> GPLGSEQQPGDRCPRHVARIIAENDPPIRCDLTLQELLSEVQVDFEPSASEVVAMEGLMDEQHFIPHDPHSKKAAVQSLVIAIKTADLLLQMIHENVKRDIRTTCIQMANESYARADIVRDSLIAASQGKYTALGKIVFHSYTNFMPVNANESEKRAWMEMLGECTSHGNKLCEMANAQVEQETRDIINIMFKNIDDVVTQTTRAMRGVFDPPDTVKALSAAAQLIRVWEHDNVINDQSVSTSSVVTAALEANENLAKALRDVSGYAEVQFNRLCLSILTSAKERIDIIYHSARSQHLACNVRMNVAQQNLATFILTNARERPNDAVIRTRRAVANTGILLFTGQHITRDALDKAAESKSVEEIVGMS

To ensure the success of lytic replication, the herpesvirus human cytomegalovirus (HCMV) expresses the immediate-early protein IE1, which acts as an antagonist of antiviral, subnuclear structures termed PML nuclear bodies (PML-NBs). IE1 interacts directly with PML, the key protein of PML-NBs, through its core domain and disrupts the dot-like multiprotein complexes thereby abrogating the antiviral effects. Structural characterization of IE1 has shown that it comprises a folded core domain (IE1CORE), which mediates the interaction with PML and is flanked by a short disordered region at the N-terminus and a longer disordered region at the C-terminus containing a SUMOylation motif and a STAT interaction site. All three IE1CORE proteins display a femur-like structure consisting of α-helices only.

Of the two ratIE1 variants, only the N-terminally truncated variant yielded protein crystals. This variant, covering residues 30 to 392, is from here-on referred to as the ratIE1CORE domain. For crystallization, surface lysine residues of ratIE1 30–392 were chemically methylated. The structure of ratIE1CORE was solved to 3.4 Å resolution with Rwork = 21.5% and Rfree = 24.6%. Initial phases were obtained with the MAD technique since any molecular replacement calculations with the previously determined rhesIE1CORE structure failed. The main chain of ratIE1CORE could be built from residues 33 to 392, and only three N-terminal residues could not be located in the electron density. In case of ratIE1CORE, the correct sequence registration has been corroborated by two additional anomalous scattering experiments, thereby rendering the possibility of registration errors highly unlikely. Thus, helix H1 is significantly shorter in ratIE1CORE, and the position of H2 is rotated by approximately 90° in comparison to humIE1CORE and rhesIE1CORE. Furthermore, a kink separates helices H5 and H6 in humIE1CORE and rhesIE1CORE, whereas ratIE1CORE contains one continuous helix termed H5/6. At the same time, ratIE1CORE has an additional helix H12 at the C-terminus in comparison to humIE1CORE and rhesIE1CORE, which consist of eleven helices in total. However, whereas the stalk and the adjacent C-terminal head region of ratIE1CORE are formed by continuous right-handed coiled-coils, this segment is interrupted by a region of left-handed coiled-coils in rhesIE1CORE and humIE1CORE.> MPFAGSELPRRPLPPAAQERDAEPRPPHGELQYLGQIQHILRCGVRKDDRTGTGTLSVFGMQARYSLRDEFPLLTTKRVFWKGVLEELLWFIKGSTNAKELSSKGVKIWDANGSRDFLDSLGFSTREEGDLGP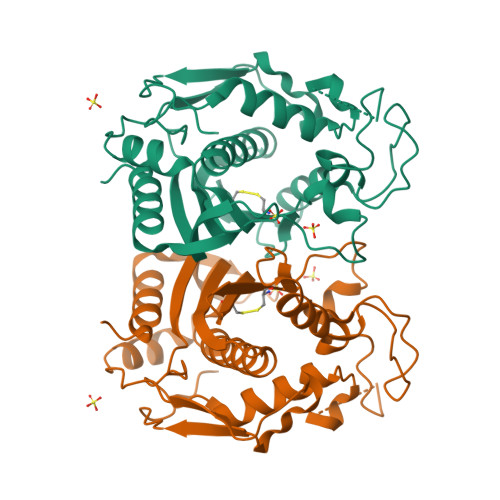VYGFQWRHFGAEYRDMESDYSGQGVDQLQRVIDTIKTNPDDRRIIMCAWNPRDLPLMALPPCHALCQFYVVNSELSCQLYQRSGDMGLGVPFNIASYALLTYMIAHITGLKPGDFIHTLGDAHIYLNHIEPLKIQLQREPRPFPKLRILRKVEKIDDFKAEDFQIEGYNPHPTIKMEMAV>GIDPFTDDFDFLSGADEAATKLDLARAYIDMGDS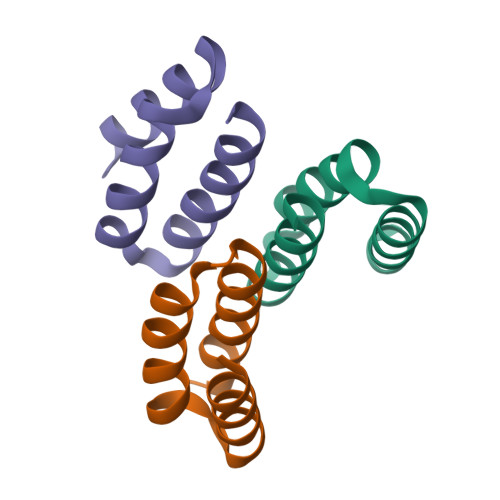EGARDILDEVLAEGNDSQQAEARELLERLA[6x]>MSDKDSKNTPQVPEKLGLSRRGFLGASAVTGAAVAATALGGAVMTRESWAQAVKESKQKIHVGPGELDDYYGFWSGGHQGEVRVLGVPSMRELMRIPVFNVDSATGWGLTNESRHIMGDSAKFLNGDCHHPHISMTDGKYDGKYLFINDKANSRVARIRLDIMKCDKMITVPNVQAIHGLRLQKVPHTKYVFANAEFIIPHPNDGKVFDLQDENSYTMYNAIDAETMEMAFQVIVDGNLDNTDADYTGRFAAATCYNSEKAFDLGGMMRNERDWVVVFDIHAVEAAVKAGDFITLGDSKTPVLDGRKKDGKDSKFTRYVPVPKNPAGCNTSSDGKYFIAAGKLSPTCSMIAIDKLPDLFAGKLADPRDVIVGEPELGLGPLHTTFDGRGNAYTTLFIDSQVVKWNMEEAVRAYKGEKVNYIKQKLDVHYQPGHLHASLCETNEADGKWLVALSKFSKDRFLPVGPLHPENDQLIDISGDEMKLVHDGPTFAEPHDCIMARRDQIKTKKIWDRNDPFFAPTVEMAKKDGINLDTDNKVIRDGNKVRVYMTSMAPAFGVQEFTVKQGDEVTVTITNI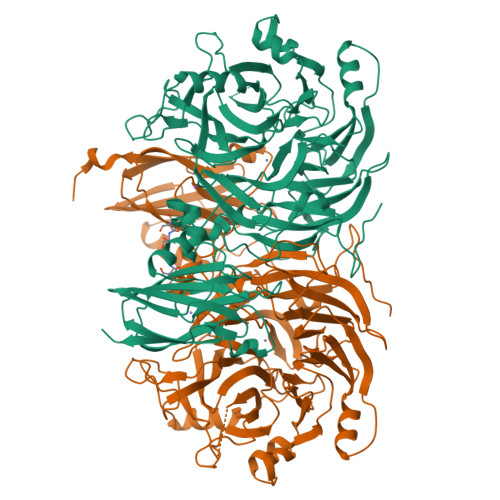DQIEDVSHGFVVVNHGVSMEISPQQTSSITFVADKPGLHWYYCSWFCHALHMEMVGRMMVEPAWSHPQFEK[2x]> DRHHHHHHGSAPDQDEIDALPGLAKQPSFRQY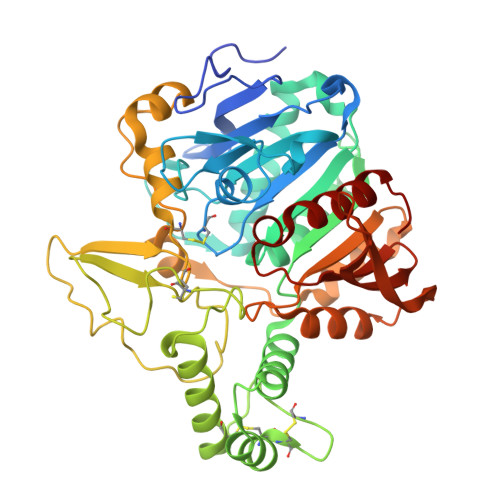SGYLRASDSKHFHYWFVESQNDPKNSPVVLWLNGGPGCSSLDGLLTEHGPFLIQPDGVTLEYNPYAWNLIANVLYIESPAGVGFSYSDDKMYVTNDTEVAENNYEALKDFFRLFPEYKDNKLFLTGESYAGIYIPTLAVLVMQDPSMNLQGLAVGNGLASYEQNDNSLVYFAYYHGLLGNRLWTSLQTHCCAQNKCNFYDNKDPECVNNLLEVSRIVGKSGLNIYNLYAPCAGGVPGRHRYEDTLVVQDFGNIFTRLPLKRRFPEALMRSGDKVRLDPPCTNTTAPSNYLNNPYVRKALHIPESLPRWDMCNFLVNLQYRRLYQSMNSQYLKLLSSQKYQILLYNGDVDMACNFMGDEWFVDSLNQKMEVQRRPWLVDYGESGEQVAGFVKECSHITFLTIKGAGHMVPTDKPRAAFTMFSRFLNKEPY>TVADKQARLMPLFKHLTALTREKLPLDQRDERLKGVGILPRGTLFSCFHARHLAEATELYVALYGAKDFNDFIHLCEQARQIVNEGMFVYAVSVAVLHREDCKGITVPPIQEVFPDRFVPAETINRANKEASNHPDQQSIVVEAEETGNILDPEYKLSYFR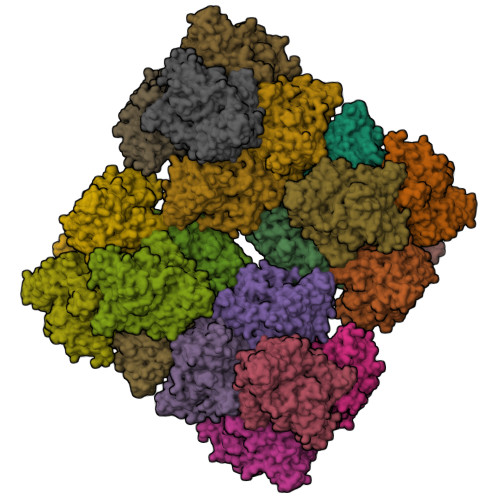EDIGINAHHWHWHIVYPATWNPTVMGKEKDRKGELFFYMHQQMCARYDSERLSNGLQRMIPFHNFDEPLEGYAPHLTSLVSGLQYASRPEGYSIHDLSDVDVQDMVRWRERILDAINMHYIVDKDNNKIPLDIEHGTDILGDIIESSDESKNVEYYGSLHNWGHVMMANITDPDHRFQENPGVMSDTSTSLRDPIFYRWHRFIDNIFQEHKKSFHPYTKEELSFPGVEVVGVSINSKTANVITTLIKESLLELSHGINFGTDQSVKVKYHHLDHEPFTYNIVVENNSGAEKHSTVRIFLAPKYDELNNKLEPDEQRRLFIELDKFFYTLTPGKNTIVRNHQDSSVTISKVRTFDQLGAGEGVSEDSTEYCSCGWPEHMLIPRGSHKGMEFELFVMLTDHDEDTVAGLSENAVCSDAVSYCGARDDRYPDKKAMGFPFDRKIEARTAAEFLTPNMGLTDIKIKFHG[12x]>[14x]MNQTLETGTTTVGITLKDAVIMATERRVTMENFIMHKNGKKLFQIDTYTGMTIAGLVGDAQVLVRYMKAELELYRLQRRVNMPIEAVATLLSNMLNQVKYMPYMVQLLVGGIDTAPHVFSIDAAGGSVEDIYASTGSGSPFVYGVLESQYSEKMTVDEGVDL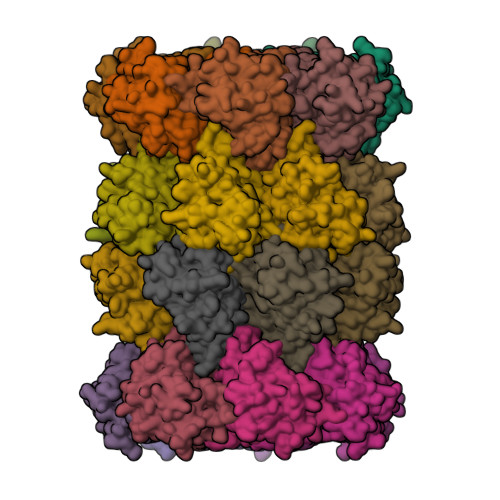VIRAISAAKQRDSASGGMIDVAVITRKDGYVQLPTDQIESRIRKLGLIL;>[14x]MQQGQMAYDRAITVFSPDGRLFQVEYAREAVKKGSTALGMKFANGVLLISDKKVRSRLIEQNSIEKIQLIDDYVAAVTSGLVADARVLVDFARISAQQEKVTYGSLVNIENLVKRVADQMQQYTQYGGVRPYGVSLIFAGIDQIGPRLFDCDPAGTINEYKATAIGSGKDAVVSFLEREYKENLPEKEAVTLGIKALKSSLEEGEELKAPEIASITVGNKYRIYDQEEVKKFL6-methoxy-4-[(methylamino)methyl]-2-(6-{4-[(2S)-4,4,4-trifluorobutan-2-yl]-4H-1,2,4-triazol-3-yl}pyridin-2-yl)-2,3-dihydro-1H-isoindol-1-one 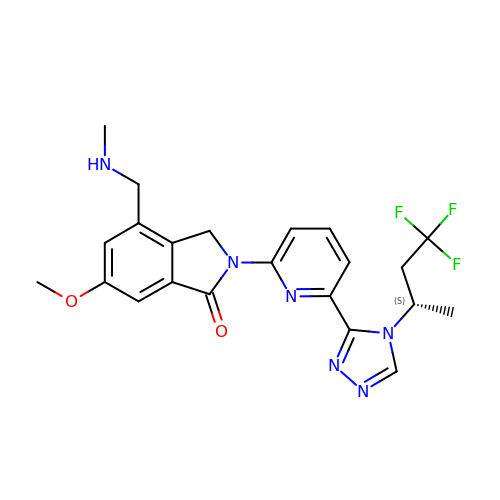| C22 H23 F3 N6 O2 | DVPICGLUATZNJY-ZDUSSCGKSA-N> MSGMLQARAVDEDTLEADYLIETPLDPARVADVMAGEQSSGTFVRVANESDALRARSRASVLRIEELEAAARPSLPNAWLERQGTPGPWRRARITLSFPLANIDANLPTLAATVAGNLYDLGEVTGVRLLSLRLPASYRARFELPRHGVAGTRALTDVKDRPMIGTIIKPNVGLSAAETAALVRELCEAGVDFIKDDEVCANPAHAPLAERVRAVMSEVRRYRERSGRPVMVAFNITDDLDAMRRHAELVEREGGSCVMASINWCGFSAIQSLRRTTPLVLHAHRNGYGMMSRDPALGMSFQAYQTLWRLSGVDHMHVHGLAGKFAQSDAEVIESARDCATPLAAGCDDAVLPAFSSGQWAGTVQATFDAVRSTDLLFMSGGGILA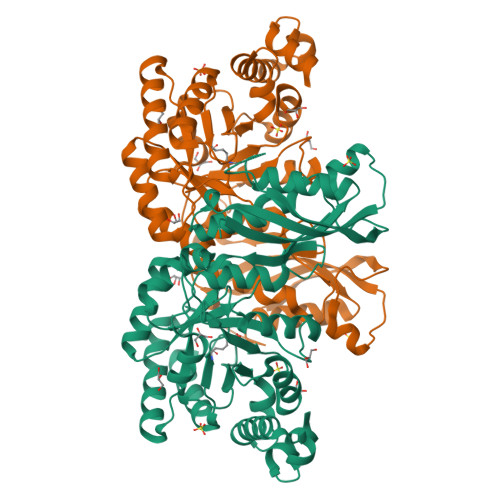HPDGPAAGVTSVRQAWAAVQAGTPLPVYAEHMPELRRALAFFGGRA> G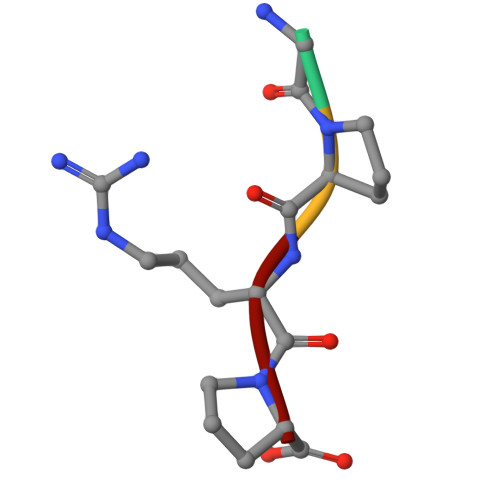PRP>MKAVQYTEIGSEPVVVDIPTPTPGPGEIL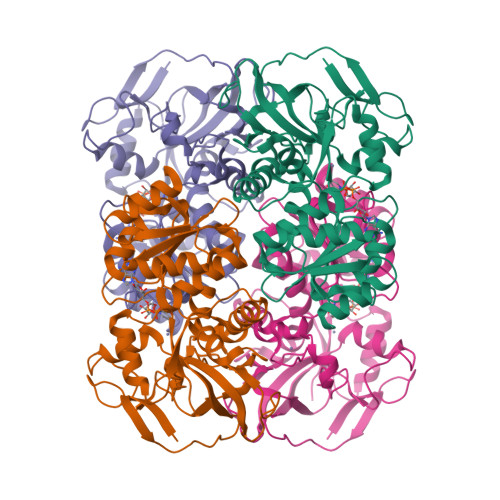LKVTAAGLCHSDITVMDMPAAQYAGGLPLTLGHEGVGTVAELGEGVTGFGVGDAVAVYGPWGCGACHACARGRENYCTRAADLGITPPGYGSPGSMAEYMIVDSARHLVPIGDLDPVAAAPLTDAGLTPYHAISRVLPLLGPGSTAVVIGVGGLGHVGIQILRAVSAARVIAVDLDDDRLALAREVGADAAVKSGAGAADAIRELTGGQGATAVFDFVGAQSTIDTAQQVVAVDGHISVVGIHAGAHAKVGFWMIPFGASVVTPYWGTRSELMEVVALARAGRLDIHTETFTLDEGPAAYRRLREGSIRGRGVVVPTSHHHHH[4x]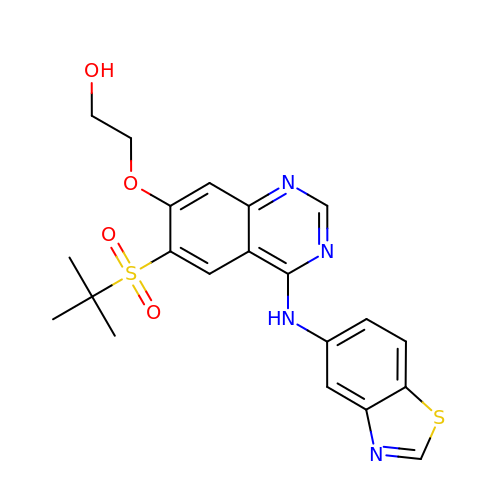2-[4-(1,3-benzothiazol-5-ylamino)-6-~{tert}-butylsulfonyl-quinazolin-7-yl]oxyethanol | C21 H22 N4 O4 S2 | UHDOJINBFLDQJM-UHFFFAOYSA-N>GPLGSGVPHEITGGNRQEKLAQLMRQFESGGLYLRTVSDHRDEFENTFMPKLDACLGHGCDERYWSSATFIQQGLNGKVHDPHADRTGLIISADARLGGFSTFDAATANVPSGLEPSQYFPGQFPKFDMMGAYQATWNEDIFSVDATAVSEQQMDELGIPDEYRSVFDFDRIQEKMAQPRLAGREVEPTEAKICYQPKDVLGIYVDVDSPASQSKARELQQAMREQGFDLPFIAYRGGAAQELASV[3x]

A recent study found that CteC, an effector from the bacterial pathogen Chromobacterium violaceum, hinders host ubiquitin (Ub) signaling pathways via installing mono-ADP-ribosylation on threonine 66 of Ub. Regarding enzyme classification, CteC belongs to the ARTC family with an R-S-E motif (R65, S97, and E220), with R65 and E220 being catalytically essential residues. The MARylation occurs on Thr66 of Ub, resulting in an ADP-ribosylated Ub derivative that is nonfunctional in a variety of Ub-related processes ultimately leading to the malfunction of host Ub system. CteC adopts a canonical mART fold with an additional insertion domain, which is needed for Ub binding and catalytic activity.

Therefore, we expressed and purified the selenomethionine-substituted CteC36–276 (SeMet-CteC36–276), crystallized it in complex with NAD+, and determined its structure at 1.87 Å via single-wavelength anomalous diffraction (SAD) phasing. The NAD+-bound SeMet-CteC36–276 crystallized in P21 21 21 space group, with three copies in one asymmetric unit. The CteC structure harbors two domains, a core mART domain with NAD+ bound and a small helical insertion domain with no apparent interaction with NAD+. The insertion domain in CteC is a small four-helical bundle present between β4 and β5, spanning from residue F157 to R194. Within the mART domain, every atom of NAD+ can be unambiguously placed in its binding pocket based on the electron density in all three copies in the asymmetric unit. Overall, NAD+ binds CteC in a bent conformation via multiple interactions. Specifically, the adenine base is primarily positioned by the π–cation interaction with the guanidinium group of the R93 side chain, with additional interactions with W95 carbonyl oxygen and R65 side chain via N6 and N7 atoms, respectively. The diphosphate group is held by the R65 side chain, with additional polar interactions of α-phosphate to N139 side chain and β-phosphate to R113 side chain. The NAM ribose is held via hydrogen bonding between C2’’ hydroxyl group and the side chains of D134 and E220. Curiously, we observed a Ca2+ ion near the NAM ribose, coordinating with C2’’ and C3’’ hydroxyl groups, D134 side chain, A135 backbone carbonyl oxygen, and three water molecules.> MKTEWPELV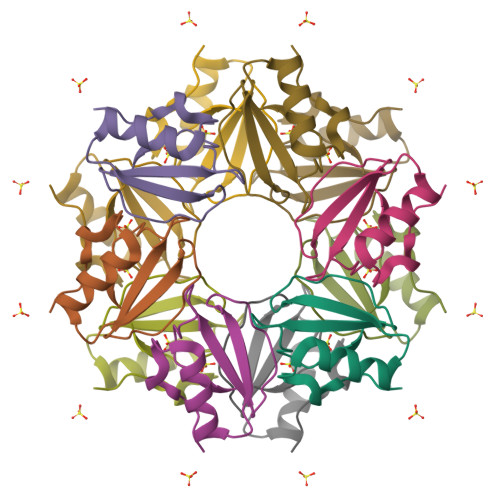GKSVEEAKKVILQDKPEAQIIVLPVGTIVTMEYRIDRVRLFVDKLDNIAQVPRVG>MHSVKLNNNYEMPIIGLGTFRSKKNDAYNAVKAALEGGY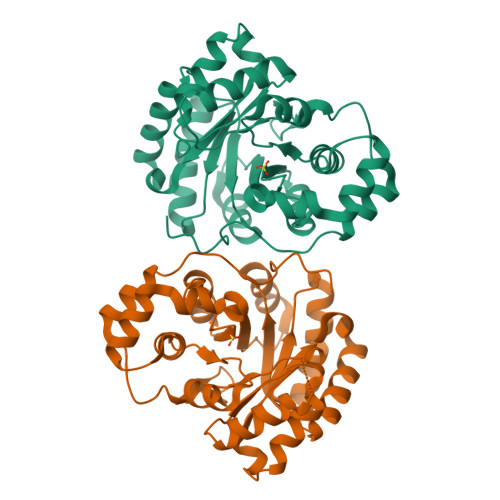RHIDTAMIYGNEEEVGRAIKDSNIPREEIFVTTKLWNTDQGYEKTLEAFNTSLKNLGLDYIDLYLIHWFKGYDNALSTYRAFETLYEEGKVKAIGVSNFNVHHLMYLMENAKIPPMVNQVETHVTLQNHFLHDYCKKNNIQLEAYAPLMSHQIKDLLSNETMAKIAKKHDKTIPQIAIRWLIEREIVVIPKSITPERIVQNFDVFDFTLDEEDMKSIRSVNTGKKIFTEFDNVDY[6x]> MSIITDVYAREVLDSRGNPTLEVEVYTESGAFGRGMVPSGASTGEHEAVELRDGDKARYGGLGTQKAVDNVNNVIAEHIIGFDVRDQQGIDRAMIALDGTPNKGKLGANA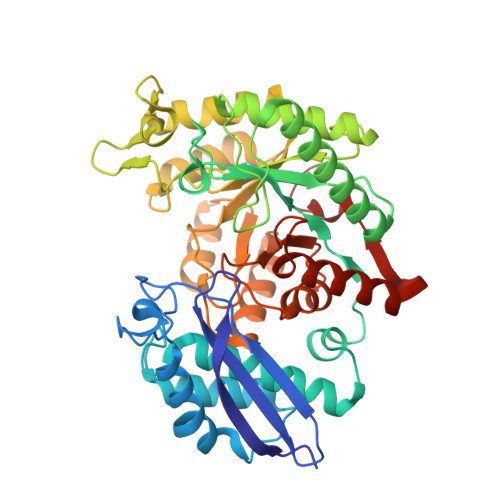ILGVSIAVARAAADYLEVPLYSYLGGFNTKVLPTPMMNIINGGSHSDAPIAFQEFMIVPAGAPTFKEALRWGAEIFHALKKILKERGLETAVGDEGGFAPRFNGTEDGVETIIKAIEAAGYVPGKDVFIGLDCASSEFYDAEHKVYGYTKFEGEGAAVRTAAEQIDYLEELVNKYPIITIEDGMDENDWDGWKALTERLGGKVQLVGDDFFVTNTAYLEKGIAEHAANSILIKVNQIGTLTETFDAIEMAKEAGYTAVVSHRSGETEDSTIADIAVATNAGQIKTGSLSRTDRIAKYNQLLRIEDQLGEVAEYRGLKSFYNLKK> GSHMDGRIYAVGGYDGSPDGHTHLNSVEAYDPETDTWSLVAPMKTRRSGVGVAVLDGRIYAVGGYDGSPDGHTHLNSVEAYDPETDTWSLVAPMKTRRSGVGVAVLDGRIYAVGGYDGSPDGHTHLNSVEAYDPETDTWSLVAPMKTRRSG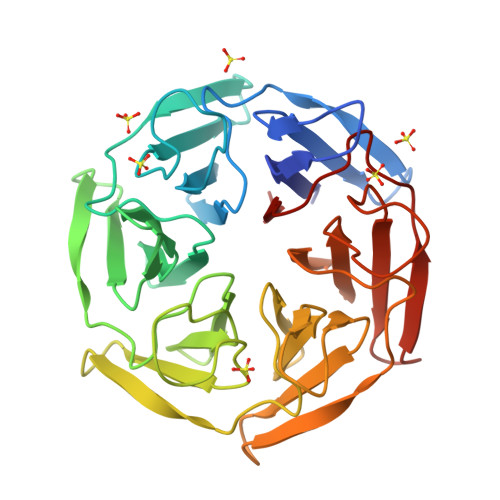VGVAVLDGRIYAVGGYDGSPDGHTHLNSVEAYDPETDTWSLVAPMKTRRSGVGVAVLDGRIYAVGGYDGSPDGHTHLNSVEAYDPETDTWSLVAPMKTRRSGVGVAVLDGRIYAVGGYDGSPDGHTHLNSVEAYDPETDTWSLVAPMKTRRSGVGVAVL>MDLHKAMGQFFDAKGNIALPPQITLAGLSELFYQSDVDGGDRHCMRYWDYSTEGGVARDYNRREINTRIKSVAARLQQVAQPGDRVAILANNSPEYLFGFIGALYAGLVPVPLYDPSEPGHADHLTAVMADAQPAIVLTNNASAAAVRRFFSALPGAQRPRIISIDSLPDTLAQSYQIPTPSMAAAAINPVDLPAFLQYTSGSTRTPAGVVLTNRSIVTNVLQIFAAAQLKTPLRLVSWLPLHHDMGIILAVFITLLGLEFEMMSPRDFIQQPKRWIDQLDRREGDNAVYAVVPNFALELAARYATPSEGLDLSAVEGLIIGSEPVTEKAVEAFA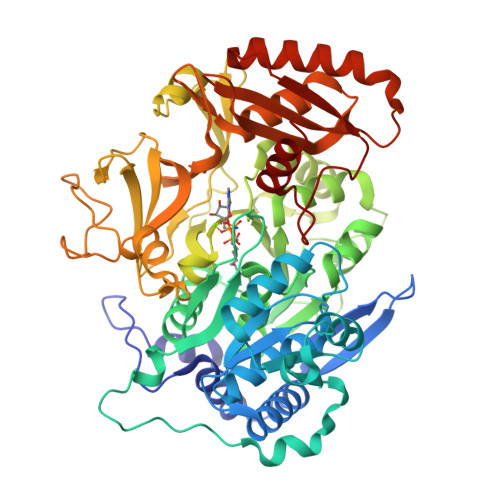ETFGPYGLNRQNMRPSYGLAEASLLVTTPQTPQRPVISYFDREQLAANRAVIVDKGDNAVALTGVGQVVRPQNLVIVDPETRTEVADGTIGELWAHGENMAAGYLDRPEDTAETFHNTLAGRLENSRAAGVPEESTKWMATGDLGVIVDGELYITGRLKDLVIIAGRNHYPQDIEYTVDHASEHIRPAAVAAFAIEGDAVEQLIILAERDLDRDPSGDAEAIDAIRAAVTEAHGVVPADIRIVAPDEILRSSSGKIARRVNKKAYQESH[4x]> VLSDFQEAVPTVVGIPDGTAVVGRSFRVSIPTDLIASSGEIIKVSAAGKEALPSWLHWNPHSHILEGLPLDTDKGVHYISVSAARLGANGSHVPQTSSVFSIEVYPEDHNEPQSVRAASSDPGEVVPSACAADEPVTVLTVILDADLTKMTPKQRIDLLNRMQSFSEVELHNMKLVPVVNNRLFDMSAFMAGPGNAKKVVENGALLSWKLGCSLNQNSVPDIRGVETPAREGAMSAQLGYPVVGWHIANKKPTLPKRLRRQIH

Dystroglycan (DG), a ubiquitous membrane receptor belonging to the glycoprotein complex associated to dystrophin, plays a crucial role in the stability of the plasma membrane, especially in skeletal muscle tissues where it is highly expressed. A single gene, DAG1, encodes for a protein precursor, which is proteolytically cleaved in two subunits, alpha-dystroglycan (α-DG), located at the extracellular side of the plasma membrane where it binds several extracellular matrix proteins, and beta-dystroglycan (β-DG), which is a transmembrane protein that interacts with dystrophin in the cytoplasm. The molecular structure of the N-terminal region of α-DG (α-DG-Nt) was later determined at high resolution by X-ray crystallography, revealing the presence of two domains, an immunoglobulin-like (Ig-like) domain and a domain similar to the small subunit ribosomal protein S6 of T. termophilus (S6 domain), connected by a flexible loop. Noteworthy, it has been shown that α-DG-Nt is necessary for recruiting LARGE and some pathological conditions that are caused by missense mutations in the DAG1 map within the α-DG-Nt.

The crystal structures of D109N and V72I have been determined to a resolution of 1.70 Å and 1.80 Å, respectively. The Asp109→Asn mutation introduces local changes on the molecular geometry that are quite evident in the final refined model. The Asn109 side chain rotates nearly 120° around Cα-Cβ with respect to the orientation held by Asp109 in the WT. The conformation assumed by Asn109 allows for the establishment of H-bonds with Lys203, Glu116 and His107. Accordingly, Asn109 is not engaged anymore in H-bonds with Ser112 and His111 as Asp109 is in WT. In addition, the H-bond network involving Asn109, Glu116 and Lys203 in D109N abolishes the interaction between Lys203 and Glu116 observed in the WT structure. In this respect, it must be emphasized that the Asp109→Asn mutation not only changes the H-bond network involving residue 109, but also modifies the local electrostatic potential, so that the interaction of Asn109 with the surrounding positively charged residues like Lys203 and Arg77 is affected. This is confirmed by the presence of two water molecules (HOH 548 and 621) absent in WT structure and coordinating Arg77, thus filling the void left by the Asn109 side-chain relocation. In details, the mutations Asp109→Asn and Thr190→Met led to a significant increase in the maximum dimensions (with Dmax increased from 90 ± 3Å for WT to 95 ± 3Å and to 100 ± 3Å for D109N and T190M respectively) and in the Rg values (from 25.20 ± 0.04Å for the WT to 26.40 ± 0.04Å and to 27.20 ± 0.04Å for D109N and T190M, respectively), suggesting a more extended shape of the two pathological mutants compared to the WT protein.>MGHHHHHHSHMDELLNRLRQTWHSTIPVSEFMQIAPLSFTDGELSVSAPLAPNINLHHTMFAGSIYTIMTLTG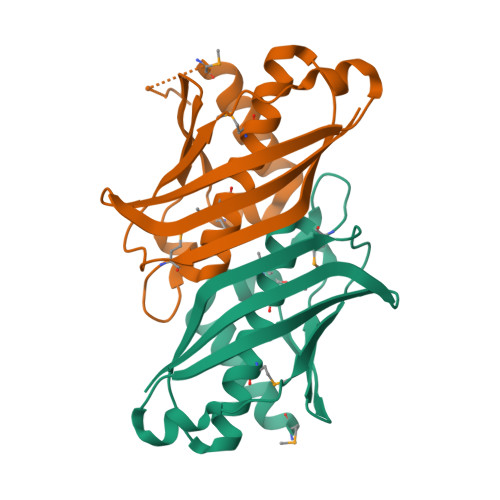WGMVWLQQQLLNVDGDIVLADAHIRYLAPVTSAPEVKVRWPDTNLSPLQRGRKAKVKLEVQLFCDGKLCAQFDGLYVSVPKM[4x]> MKTSSLRKSVCSDLLTLFNSPHSALPSLLVSGMPEWQ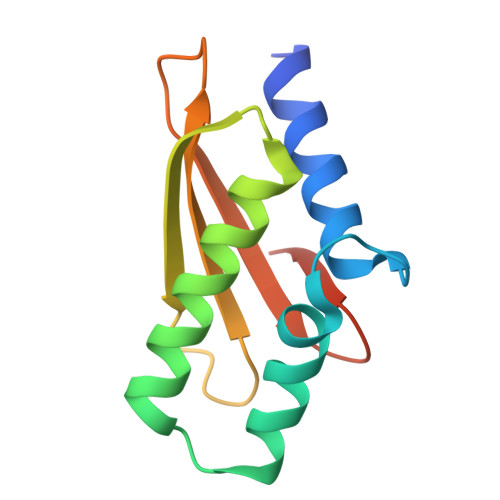VHNPSDKHLQSWYCRQLRSALLFHEPRIAALQVNLKEAYCHTLAISLEIMLYHDDEPLTFDLVWDNGGWRSATLENVS> LEEKKVCQGTSNKLTQLGTFEDHFLSLQRMFNNCEVVLGNLEITYVQRNYDLSFLKTIQEVAGYVLIALNTVERIPLENLQIIKGNMYYENSYALAVLSNYDANKTGLKELPMRNLQEILHGAVRFSNNPALCNVESIQWRDIVSSDFLSNMSMDFQNHLGSCQKCDPSCPNGSCWGAGEENCQKLTKIICAQQCSGRCRGKSPSDCCHNQCAAGCTGPRESDCLVCRKFRDEATCKDTCPPLMLYNPTTYQMDVNPEGKYSFGATCVKKCPRNYVVTDHGSCVRACGADSYEMEEDGVRKCKKCEGPCRKVCNGIGIGEFKDSLSINATNIKHFKNCTSISGDLHILPVAFRGDSFTHTPPLDPQELDILKTVKEITGFLLIQAWPENRTDLHAFENLEIIRGRTKQHGQFSLAVVSLNITSLGLRSLKEISDGDVIISGNKNLCYANTINWKKLFGTSGQKTKIISNRGENSCKATGQVCHALCSPEGCWGPEPRDCVS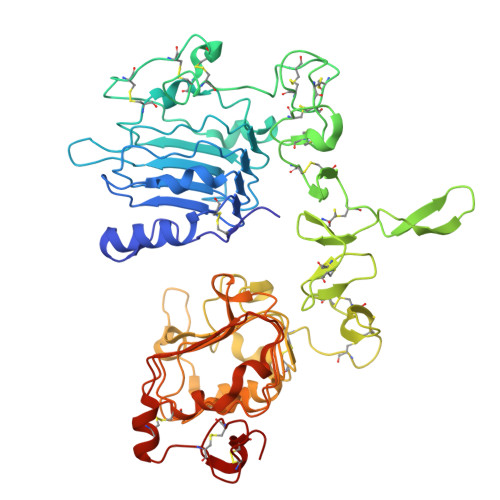H>[2x]MEIKETYDFSSIVDLWNKNIGTVYPMNLELFKQNYINDRQRKKIMGAFNGEILIGFVIYKQWTYKSGSLKPNHKIGYINSIIVDINFRHQGIGTKLLDAAEEELINSGVKILRCGSDTYHFFPGIPLECLPSEEFFLVRGYKMQDYFYDLIGDVSKVDFKKPSIKDGFKVNVMKPEDRKGLFEFLE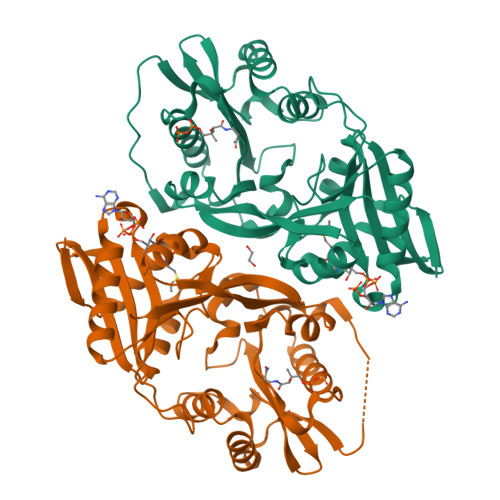KSFSGRWLEEFIEFFQVGMKERDIVLIKYKTSVIGFSHIYDNKSSFIGPPIYWKALLGHNYGGLGPIGIDKTYRKQGLGRLLLYESLQILKKREVKKMVIDWTEKDIINFYGRFNFMPWKAYRKATKEVKDGKGGGHHHHHH Rebaudioside 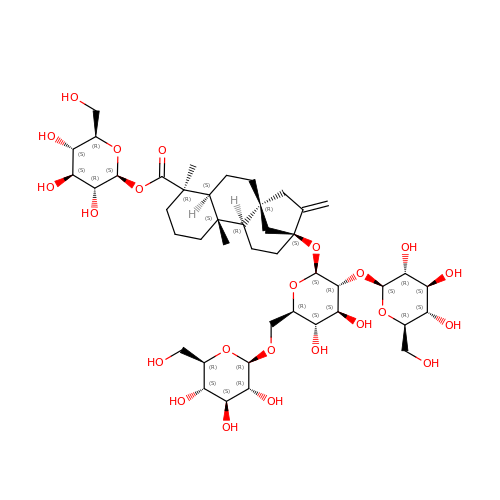A2 | C44 H70 O23 | SPYZRRVRFHDMJY-QMEMPQSWSA-N> MKFSVIVPTYNSEKYITELLNSLAKQDFPKTEFEVVVVDDCSTDQTLQIVEKYRNKLNLKVSQLETNSGGPGKPRNVALKQAEGEFVLFVDSDDYINKETLKDAAAFIDEHHSDVLLIKMKGVNGRGVPQSMFKETAPEVTLLNSRIIYTLSPTKIYRTALLKDNDIYFPEELKSAEDQLFTMKAYLNANRISVLSDKAYYYATKREGEHMSSAYVSPEDFYEVMRLIAVEILNADLEEAHKDQILAEFLNRHFSFSRTNGFSLKVKLEEQPQWINALGDFIQAVPERVDALVMSKLRPLLHYARAKDIDNYRTVEESYRQGQYYRFDIVDGKLNIQFNEGEPYFEGIDKLVPRGSAAAALEHHHHHH

In this article we describe the crystal structure of TarS, an enzyme responsible for the glycosylation of wall teichoic acid polymers of the S. aureus cell wall, a process that has been shown to be specifically responsible for methicillin resistance in MRSA. TarS possesses a catalytic domain with a canonical GTA fold (one of two distinct A/B folds characteristic of nucleotide-sugar dependent glycosyltransferases) consisting of two closely associated α/β/α sandwich Rossmann motifs that abut and form a continuous central β-sheet. TarS possesses a D(91)XDD motif with aspartates coordinating a metal cation, a feature that is typical of the GTA superfamily. Altogether, TarS features a novel architecture with closely-associated trimerization domains connected by a linker region to three protruding catalytic domains that face away from each other.

Our analysis of the enzymatic mechanism of TarS was facilitated by the capture of various TarS1-349 structures encapsulating the catalytic domain in complex with metal and substrates. These include the native structure with bound Mn2+ (free enzyme), the UDP-GlcNAc bound structure in the presence and absence of Mn2+ (the binary Michaelis complex), and the UDP bound structure with Mn2+ (product complex). Native and UDP bound structures were also obtained to similar resolution. The structures of native and UDP bound TarS1-349 were similar to that obtained for the lower resolution UDP bound full-length TarS (overall main chain root mean squared deviation (rmsd) of 0.56 Å over 335 atom pairs), with minor differences in the linker region (320–349). Based on these observations it may be inferred that in the native structure, the SA loop is disordered allowing binding of UDP-GlcNAc, upon which the CS loop moves closer to the active site center and the SA loop becomes ordered, occluding the active site channel. Trapped sulfates from our crystallization condition were also observed in the TarS1-349 structure along two basic grooves leading into the active site centre, potentially indicating where the phosphates of the acceptor polyRboP may be bound. Kinetic parameters for wild-type and TarS1-349 constructs were similar, indicating that the trimerization domain appears to be dispensable for UDP-GlcNAc hydrolysis activity. The results show that although TarS1-349, lacking a trimerization domain, retains some processivity (133 ± 14), its Pintr is reduced compared to wild-type (2400 ± 260) indicating that oligomerization does appear to contribute to TarS processivity.>[4x]MTAPTVPVALVTGAAKRLGRSIAEGLHAEGYAVCLHYHRSAAEA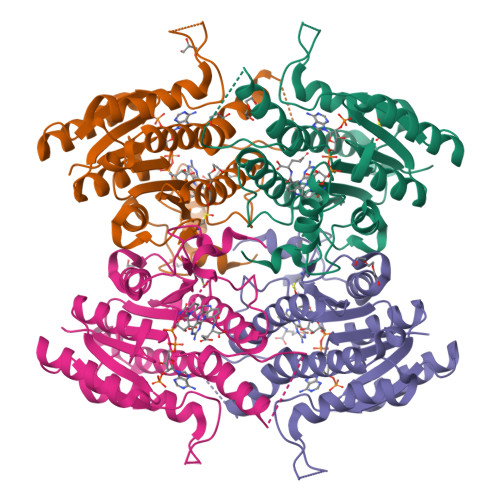NALSATLNARRPNSAITVQADLSNVATAPVSGADGSAPVTLFTRCAELVAACYTHWGRCDVLVNNASSFYPTPLLRNDEDGHEPCVGDREAMETATADLFGSNAIAPYFLIKAFAHRVAGTPAKHRGTNYSIINMVDAMTNQPLLGYTIYTMAKGALEGLTRSAALELAPLQIRVNGVGPGLSVLVDDMPPAVWEGHRSKVPLYQRDSSAAEVSDVVIFLCSSKAKYITGTCVKVDGGYSLTRA1-[5-[3,4-bis(fluoranyl)-2-[2-(1,3,5-trimethylpyrazol-4-yl)ethoxy]phenyl]-1-methyl-indazol-3-yl]-~{N},~{N}-dimethyl-methanamine 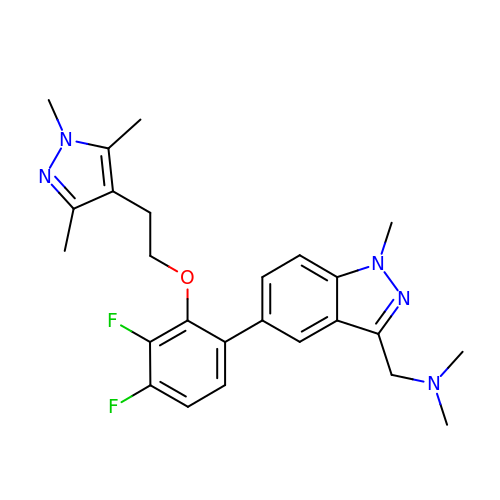| C25 H29 F2 N5 O | SOXNKJCQBRQUMS-UHFFFAOYSA-N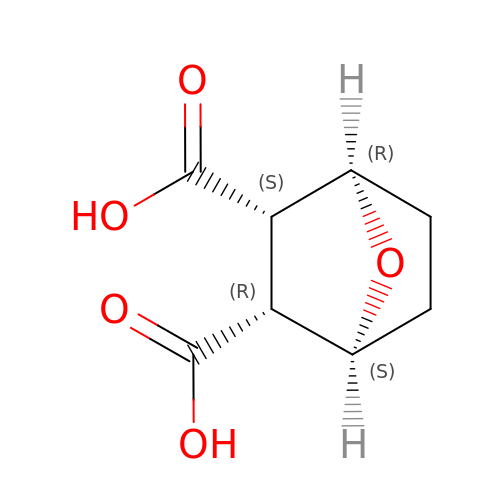(1R,2S,3R,4S)-7-oxabicyclo[2.2.1]heptane-2,3-dicarboxylic acid | C8 H10 O5 | GXEKYRXVRROBEV-FBXFSONDSA-N> SMTNVQILHGDLSPDLCDLARASELVGWDIETSGLDWRNGQIGTCQLAIGDSVAVVVLGDDDHPQGLCDLLADDGVRKIFHHAPFDIRFMAQQWDCKPRNLACTKIASKVLNPSAEHATHSLKPLLKATLGVDIDKGQQQSSWTTGVLTAEQMSYAVSDVVYLSELYSQLRAQCLDKGVLQAVENAYSFLPVWVELQRRGIEDVFAY

Dinucleases of the DEDD superfamily, such as oligoribonuclease, Rexo2 and nanoRNase C, catalyze the essential final step of RNA degradation, the conversion of di- to mononucleotides. The active sites of these enzymes are optimized for substrates that are two nucleotides long, and do not discriminate between RNA and DNA. The active sites invariably consist of (i) a catalytic DEDDh/y-containing core for divalent cation coordination and catalysis, (ii) a leucine residue that wedges between the two bases of the substrates and (iii) a 5′-phosphate cap that coordinates the 5′ phosphate of the dinucleotides. Here, we identified a novel DEDD subfamily, members of which function as dedicated deoxydinucleases (diDNases) that specifically hydrolyze single-stranded DNA dinucleotides in a sequence-independent manner.

To understand the molecular basis for the specificity of dimeric NrnC homologs toward DNA substrates, we determined a set of crystal structures of diDNases: (i) a complex of diDNaseNoc with dpGG to 1.55 Å and (ii) diDNase from Rhodococcus (diDNaseRho) in its apo state (1.72 Å resolution) and in complex with dpGG (2 Å resolution). In both structures, the 5′ phosphate of dpGG forms a set of salt bridges and hydrogen bonds with the side chains of conserved residues K104, H80 and Y206, the latter of which is contributed by the second protomer, and the main-chain nitrogen of L121 (per diDNaseNoc residue numbering). The side chain of Y206 also forms a π–π stacking interaction with the 5′ base of dpGG. In diDNaseNoc-dpGG, the side chain of the conserved residue Ser120 engages in another hydrogen bond with the 5′ phosphate, whereas in diDNaseRho-dpGG, it points away from the phosphate. Additionally, L34 splays the two bases of the substrate apart in the same manner as leucine wedges in dinucleases NrnC and Orn. In the diDNaseNoc-dpGG structure, the C-terminus of protomer B is pushed deeper into the active site of protomer A than that observed in the NrnCBh-pGG structure, creating relatively less space for the 5′ end of the substrate. In NrnCBh-pGG, the side chain of residue H205 forms a moderately strong hydrogen bond with a distance of 2.9 Å with the ether oxygen of the 5′ ribose, while in diDNaseNoc-dpGG the side chain of Y206 repulses the ether oxygen of 5′ deoxyribose, pushing the entire nucleotide away. Coordination of the ether oxygen in diDNaseNoc-dpGG is restored by the side chain of residue H81, which donates a hydrogen from the other side of the substrate. The third discriminatory feature is the apparent restricted movement of the side chain of F84 in diDNaseNoc, which engages in a perpendicular T-shaped stacking with the benzene ring of F88. However, mutating F88 to an isoleucine residue alone or in combination with H81F/Y206H in diDNaseNoc resulted in significant loss of DNase activity without an increase in activity on diribonucleotides.> SPSAEECGYSDRVRSMTLGNSTITTQESANVVVGYGEWPSYLSDREATAEDQPTQPDVATCRFYTLESVQWE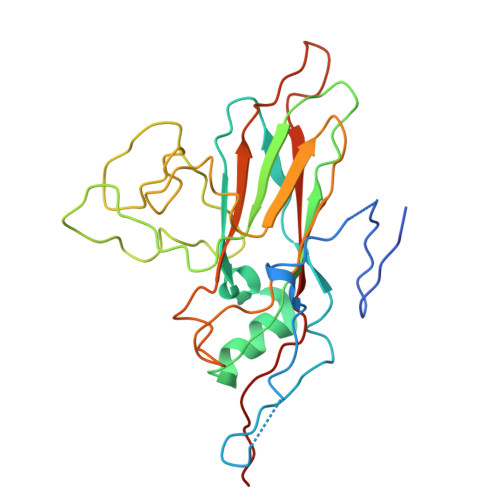KTSPGWWWKFPEALKNMGLFGQNMHYHYLGRAGYTIHVQCNASKFHQGCLLVVCVPEAEMGCADTDTTFPATELTTEDTPHVFTSDSITGKKVQAAVCNAGMGVGVGNLTIFPHQWINLRTNNSATIVIPYINSVPMDNMFRHYNFTLMIIPFAPLNFTDGATAYVPITVTIAPMYAEYNGLRLASTQ>[4x]MIERRKIAVIGSGQIGGNIAYIVGKDNLADVVLFDIAEGIPQGKALDITHSMVMFGSTSKVIGTNDYADISGSDVVIITASIPGRPKDDRSELLFGNARILDSVAEGVKKYCPNAFVICITNPLDVMVSHFQKVSGLPHNKVCGMAGVLDSSRFRTFIAQHFGVNASDVSANVIGGHGDGMVPATSSVSVGGVPLSS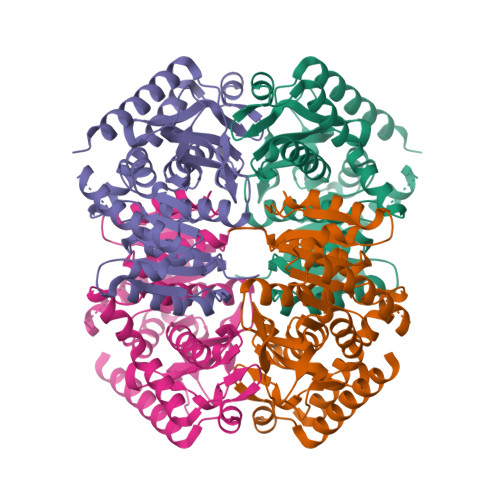FIKQGLITQEQIDEIVCHTRIAWKEVADNLKTGTAYFAPAAAAVKMAEAYLKDKKAVVPCSAFCSNHYGVKGIYMGVPTIIGKNGVEDILELDLTPLEQKLLGESINEVNTISKVLDNAPAAGA>[4x]MSKVLIVFGSSTGNTESIAQKLEELIAAGGHEVTLLNAADASAENLADGYDAVLFGCSAWGMEDLEM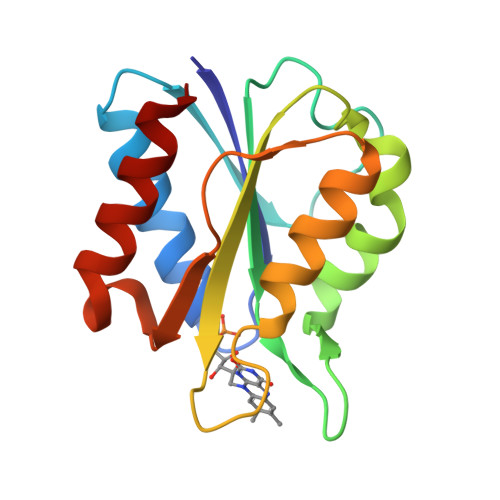QDDFLSLFEEFDRIGLAGRKVAAFASGDQEYEHFCGAVPAIEERAKELGATIIAEGLKMEGDASNDPEAVASFAEDVLKQL> MPLDPVIQQVLDQLNRMPAPDYKHLSAQQFRSQQSLFPPVKKEPVAEVREFDMDLPGRTLKVRMYRPEGVEPPYPALVYYHGGSWVVGDLETHDPVCRVLAKDGRAVVFSVDYRLAPEHKFPAAVEDAYDALQWIAERAADFHLDPARIAVGGDSAGGNLAAVTSILAKER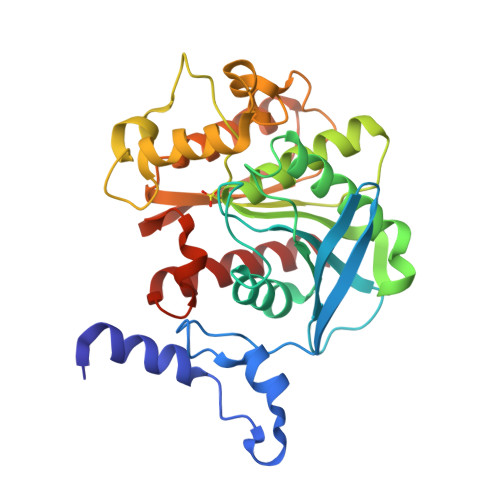GGPALAFQLLIYPSTGYDPAHPPASIEENAEGYLLTGGMMLWFRDQYLNSLEELTHPWFSPVLYPDLSGLPPAYIATAQYDPLRDVGKLYAEALNKAGVKVEIENFEDLIHGFAQFYSLSPGATKALVRIAEKLRDALA>MIALSANAFETTTPPEPPQFPAEGKINYVARDTILEFKALPSYSEPDWITEKFEKAGKLPPLKERLPEEPLVYKTGNMPDGVGVYGDTMRHVVGGRPEGWNYIAGQSQGWGGIDIALSECLTRTAPLFQVDAKDTEPLPNLAKSWEWSEDGHTLTMHLVKGAKWSDGEAFNADDVMFYWEDAVVDPNVSPLGGGASPEAFGEGTTLKKIDDYTVEWTFKAAFPKQYLYTMAYPSFCPGPSHILKPQHPKYSKNTYNQFKNAFPPEYMNMPVMGAWVPVSYRPDDLIVLRRNPYYWKVDEKGQQLPYLNEVHYKLSTWADRDVQAVAGSGDFSNLEQPENFVASLKRAADPNAPARLAFGPRLIGYNLQMNFSANGWGNPDERGQAIRELNRNEVFRQAVTSALDRKAIGDSLVKGPFTAIYPGGISSGTSFYDRASTVYYPFNLEGAKAALASIGLKDTDGDGFLNFPKETLGGRNVEITLLVNNGYATDKSLAEGLVGQMAKLGLRVVIHSLDSNQRDAAHYGGQFDWLVRRNSTELSSVVQNTEQLAPVGPRTSWNH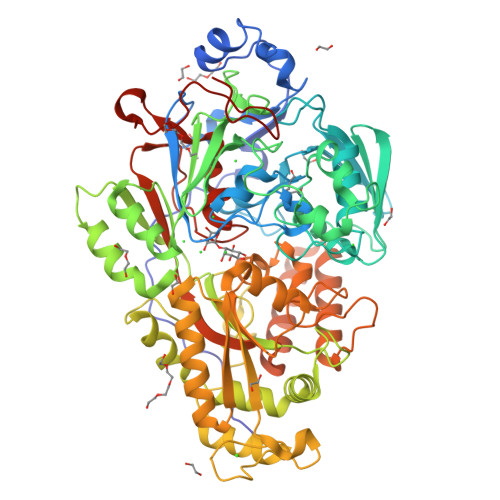RSPEGKELDLMPFEKEMADIVRKFISSQDNAERADLMKQYQKVYTQNLYTIGLTEYPGALIVNKRFSNVPQGTPIFMFNWAEDAIIRERLWVAADKQGKYELFPQQLPGKPGEGGPINHHHHHH[4x]>[4x]ANSKEVKKRASSFEWFGSNESGAEFGSGNIPGVEGTDYTFPNTTA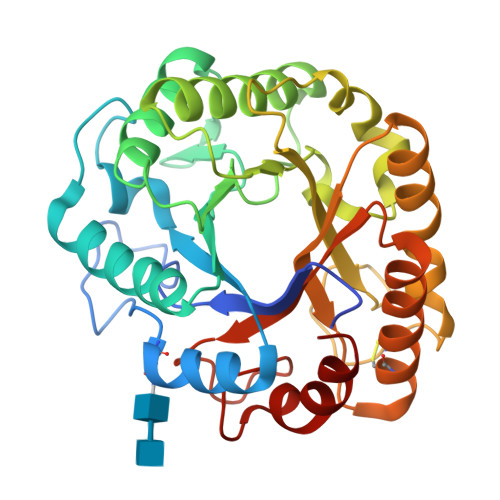IQILIDAGMNIFRVPFLMERMIPTEMTGSLDTAYFEGYSEVINYITGKGAHAVVDPHNFGRYYGTPISSTSDFQTFWSTLASQFKSNDLVIFDTNNEYHDMDESVVVALNQAAIDGIRDAGATTQYIFVEGNAYSGAWTWTTYNTAMVNLTDPSDLIVYEMHQYLDSAGSGTSDQCVSSTVGQERVVDATTWLQSNGKLGILGEFAGGANSVCEEAVEGMLDYLAENSDVWLGASWWSAGPWWQDYIYSMEPPNGIAYESYLSILETYF>VTNVGEDGEPGETEPRHALSPVDMHVHTDVSFLLDRFFDVETLELSNLTGSPATHVLDPFGSTAQLAWARLLNTCTYFFSDLELSIQFKFTTTPSSVGEGFVWVKWFPVGAPTKTTDAWQLEGGGNSVRIQQLAVAGMSPTVVFKIAGSRSQACGFSVPYTSMWRVVPVFYNGWGAPTKEKATYNWLPGAHFGSILLTSDAHDKGGCYLRYRFPRANMYCPRPIPPAFTRPADKTRHKFPTNINKQ[60x];>[60x]DKKTEETTNIEDRIETTVVGVTIINSQGSVGTTYCYSKPDGRPPSTVSDPVTRLGPTLSRHYTFKVGEWPHSQSHGHAWICPLPSDKLKKMGSFHEVVKAHHLVKNGWDVVVQVNASFAHSGALCVAAVPEYEHTHEKALKWSELEEPAYTYQQLSVFPHQLLNLRTNSSVHLVMPYIGPGPTTNLTLHNPWTIVILILSELTGPGQTVPVTMSVAPIDAMVNGPLPNPE;>[60x]APIRVVSVPESDSFMSSVPDNSTPLYPKVVVPPRQVPGRFTNFIDVAKQTYSFCSISGKPYFEVTNTSGDEPLFQMDVSLSAAELHGTYVASLSSFFAQYRGSLNFNFIFTGAAATKAKFLVAFVPPHSAAPKTRDEAMACIHAVWDVGLNSAFSFNVPYSSPADFMAVYSAEATVVNVSGWLQVYALTALTSTDIAVNSKGRVLVAVSAGPDFSLRHPVDLPDKQ;>[60x]GAGTSTPTTGNQNMSGNSGSIVQNFYMQQYQNSIDADLGDNVISPEGQGSNTSSSTSSSQSSGLGGWFSSLLNLGTKLLA

Equine rhinitis A virus (ERAV) is closely related to FMDV. The generalized picornavirus capsid is built from 60 copies of each of four structural proteins (VP1 to VP4), which are produced by cleavage of a single polyprotein by viral proteases (for a review, see reference 16). VP1 to VP3 each comprise an eight-stranded beta sandwich and form the three quasi-equivalent conformers required to build a capsid with a pseudo-T=3 surface lattice. Using cryo-electron microscopy (cryo-EM) and single particle image processing, we have determined the structure of native ERAV virions, together with the structure of a massively expanded, empty ERAV particle with large pores through the capsid layer.

The two structures reported here were solved from a single cryo-EM data set. A data set of each type (822 small and 663 large) was collected, and a structure for each was determined using single particle image processing and icosahedral averaging. The smaller particles generated a structure that, at least at the intermediate resolution of our map, is indistinguishable from previous X-ray structures of mature ERAV, while the large particles generated an expanded structure unlike any seen for any picornavirus capsid to date. As expected, the coordinates fit into our native (small) structure extremely well as a single intact unit, confirming that the smaller structure is of the native virion. However, it is tempting to speculate that the polyanionic genomic RNA must play a role, and this seems plausible given the amounts of electron density for encapsidated RNA seen in the two structures. Shown in Fig. 5a is a central, 40-Å-thick slab through the structure of the native ERAV particle, which shows that the volume encapsidated by the protein shell is full of density that we attribute to the ∼8-kb single-stranded genomic RNA packaged in the mature virion. For ERAV, which is very similar in structure to FMDV, the X-ray structures of both the native virion and low-pH-induced empty particle are extremely similar, with a root mean square deviation between the structures of only ∼0.9 Å (15).> MNVYDDVLDATVVSHSLATHFTTSDYEELLVVRTNILSVYRPTRDGKLYLTDEFKFHGLITDIGLIPQKDSPLSCLLLCTGVAKISILKFNTLTNSIDTLSLHYYEGKFKGKSLVELAKISTLRMDPGSSCALLFNNDIIAFLPFHVNKNDDDEEEEDEDENIDDSELIHSMNQKSQGTNTFNKRKRTKLGDKFTAPSVVLVASELYEGAKNIIDIQFLKNFTKPTIALLYQPKLVWAGNTTISKLPTQYVILTLNIQPAESATKIESTTIAFVKELPWDLHTIVPVSNGAIIVGTNELAFLDNTGVLQSTVLLNSFADKELQKTKIINNSSLEIMFREKNTTSIWIPSSKSKNGGSNNDETLLLMDLKSNIYYIQMEAEGRLLIKFDIFKLPIVNDLLKENSNPKCITRLNATNSNKNMDLFIGFGSGNALVLRLNNLKSTIETREAHNPSSGTNSLMDINDDDDEEMDDLYADEAPENGLTTNDSKGTVETVQPFDIELLSSLRNVGPITSLTVGKVSSIDDVVKGLPNPNKNEYSLVATSGNGSGSHLTVIQTSVQPEIELALKFISITQIWNLKIKGRDRYLITTDSTKSRSDIYESDNNFKLHKGGRLRRDATTVYISMFGEEKRIIQVTTNHLYLYDTHFRRLTTIKFDYEVIHVSVMDPYILVTVSRGDIKIFELEEKNKRKLLKVDLPEILNEMVITSGLILKSNMCNEFLIGLSKSQEEQLLFTFVTADNQIIFFTKDHNDRIFQLNGVDQLNESLYISTYQLGDEIVPDPSIKQVMINKLGHDNKEEYLTILTFGGEIYQYRKLPQRRSRFYRNVTRNDLAITGAPDNAYAKGVSSIERIMHYFPDYNGYSVIFVTGSVPYILIKEDDSTPKIFKFGNIPLVSVTPWSERSVMCVDDIKNARVYTLTTDNMYYGNKLPLKQIKISNVLDDYKTLQKLVYHERAQLFLVSYCKRVPYEALGEDGEKVIGYDENVPHAEGFQSGILLINPKSWKVIDKIDFPKNSVVNEMRSSMIQINSKTKRKREYIIAGVANATTEDTPPTGAFHIYDVIEVVPEPGKPDTNYKLKEIFQEEVSGTVSTVCEVSGRFMISQSQKVLVRDIQEDNSVIPVAFLDIPVFVTDSKSFGNLLIIGDAMQGFQFIGFDAEPYRMISLGRSMSKFQTMSLEFLVNGGDMYFAATDADRNVHVLKYAPDEPNSLSGQRLVHCSSFTLHSTNSCMMLLPRNEEFGSPQVPSFQNVGGQVDGSVFKIVPLSEEKYRRLYVIQQQIIDRELQLGGLNPRMERLANDFYQMGHSMRPMLDFNVIRRFCGLAIDRRKSIAQKAGRHAHFEAWRDIINIEFSMRSLCQGK;> MSLIHPDTAKYPFKFEPFLRQEYSFSLDPDRPICEFYNSREGPKSCPRGPLCPKKHVLPIFQNKIVCRHWLRGLCKKNDQCEYLHEYNLRKMPECVFFSKNGYCTQSPDCQYLHIDPASKIPKCENYEMGFCPLGSSCPRRHIKKVFCQRYMTGFCPLGKDECDMEHPQFIIPDEGSKLRIKRDDEINTRKMDEEKERRLNAIINGEV;> MTYKYNCCDDGSGTTVGSVVRFDNVTLLIDPGWNPSKVSYEQCIKYWEKVIPEIDVIILSQPTIECLGAHSLLYYNFTSHFISRIQVYATLPVINLGRVSTIDSYASAGVIGPYDTNKLDLEDIEISFDHIVPLKYSQLVDLRSRYDGLTLLAYNAGVCPGGSIWCISTYSEKLVYAKRWNHTRDNILNAASILDATGKPLSTLMRPSAIITTLDRFGSSQPFKKRSKIFKDTLKKGLSSDGSVIIPVDMSGKFLDLFTQVHELLFESTKINAHTQVPVLILSYARGRTLTYAKSMLEWLSPSLLKTWENRNNTSPFEIGSRIKIIAPNELSKYPGSKICFVSEVGALINEVIIKVGNSEKTTLILTKPSFECASSLDKILEIVEQDERNWKTFPEDGKSFLCDNYISIDTIKEEPLSKEETEAFKVQLKEKKRDRNKKILLVKRESKKLANGNAIIDDTNGERAMRNQDILVENVNGVPPIDHIMGGDEDDDEEEENDNLLNLLKDNSEKSAAKKNTEVPVDIIIQPSAASKHKMFPFNPAKIKKDDYGTVVDFTMFLPDDSDNVNQNSRKRPLKDGAKTTSPVNEEDNKNEEEDGYNMSDPISKRSKHRASRYSGFSGTGEAENFDNLDYLKIDKTLSKRTISTVNVQLKCSVVILNLQSLVDQRSASIIWPSLKSRKIVLSAPKQIQNEEITAKLIKKNIEVVNMPLNKIVEFSTTI;> MDGHNQNQYQNQNQIQQSQQPPLKKYVTQRRSVDVSSPYINLYYNRRHGLPNLVVEPETSYTIDIMPPNAYRGRDRVINLPSKFTHLSSNKVKHVIPAIQWTPEGRRLVVATYSGEFSLWNASSFTFETLMQAHDSAVTTMKYSHDSDWMISGDADGMIKIWQPNFSMVKEIDAAHTESIRDMAFSSNDSKFVTCSDDNILKIWNFSNGKQERVLSGHHWDVKSCDWHPEMGLIASASKDNLVKLWDPRSGNCISSILKFKHTVLKTRFQPTKGNLLMAISKDKSCRVFDIRYSMKELMCVRDETDYMTLEWHPINESMFTLACYDGSLKHFDLLQNLNEPILTIPYAHDKCITSLSYNPVGHIFATAAKDRTIRFWTRARPIDPNAYDDPTYNNKKINGWFFGINNDINAVREKSEFGAAPPPPATLEPHALPNMNGFINKKPRQEIPGIDSNIKSSTLPGLSI

Most eukaryotic messenger RNAs (mRNAs) are processed at their 3′ end by the cleavage and polyadenylation specificity factor (CPF/CPSF). CPF mediates the endonucleolytic cleavage of the pre-mRNA and addition of a polyadenosine (poly(A)) tail, which together define the 3′ end of the mature transcript. In the yeast Saccharomyces cerevisiae, CPF is assembled into a 14-subunit (∼850 kDa) complex, which is organized into three enzymatically distinct and interconnected modules: the polymerase, nuclease, and phosphatase modules (Casañal et al., 2017). The nuclease module contains the endonuclease Ysh1, the pseudo-nuclease Cft2, and the multidomain protein Mpe1 (orthologs of human CPSF73, CPSF100, and RBBP6, respectively).

To determine the architecture of the polymerase module-Cft2-Mpe1-RNA complex, we carried out single-particle cryo-EM. We used a truncated version of Cft2 (Cft2(S), residues 1–720), which is missing the disordered C-terminal region but still interacts with CPF (Kyburz et al., 2003). We obtained a map of this complex at an overall resolution of 2.8 Å. This map contained density for the polymerase module and a short region of Cft2 but not for Mpe1, the precleaved CYC1 RNA, Fip1, or Pap1 despite their presence in the cryo-EM specimen. We built an atomic model of a conserved region of Cft2 that interacts with the polymerase module and is homologous to the human CPSF100 PIM (Zhang et al., 2020). We thus refer to this region of Cft2 (residues 525–562) as the yeast polymerase module interacting motif (yPIM). The yPIM adopts an arrangement on the polymerase module that is highly similar to its human counterpart on the mPSF. Conserved aromatic residues in the yPIM (F537, Y549, and F558) stabilize its interaction with the polymerase module by inserting into the hydrophobic pockets in Cft1 and Pfs2. Mutation of these conserved residues strongly impairs the Cft2 interaction with the polymerase module. A cluster of crosslinks confirms that the yPIM binds Cft1 in the groove between beta-propellers 1 and 3 near the Cft1 helical bundle.>MSLAEPRYKADIGGGSLKLPESRIIAGLLLEGVTEDQWRHAIEVENVLQRRSPGTAKRQSSLMRNRLETMGPELWQMVRDGSTQVAIQAVFAAAIKHSTLLGDFLDLVVRDQFRMFRPDLPRKMWDQYLEQCRNRDPLMPVWQDSTANKLADCVYRILVEVGYITDSKTYRL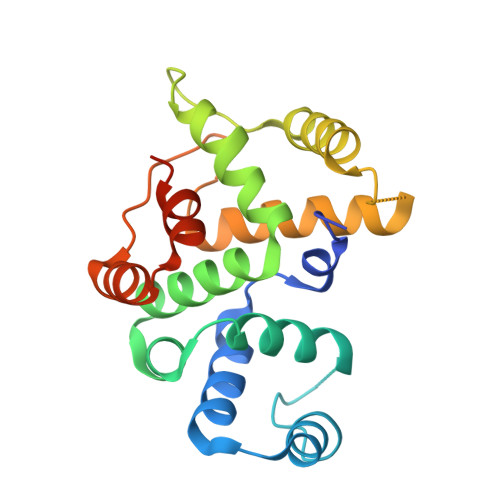KSVRISGEVMSYLRENNEQYVIRCIQVSIEGHHHHHH[2x]>[3x]GSPSSQGQHKHKYHFQKTFTVSQAGNCRIMAYCDALSCLVISQPSPQASFLPGFGVKMLSTANMKSSQYIPMHGKQIRGLAFSSYLRGLLLSASLDNTIKLTSLETNTVVQTYNAGRPVWSCCWCLDEANYIYAGLANGSILVYDV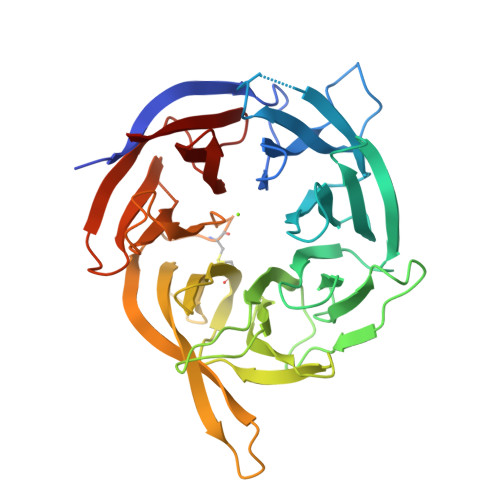RNTSSHVQELVAQKARCPLVSLSYMPRAASAAFPYGGVLAGTLEDASFWEQKMDFSHWPHVLPLEPGGCIDFQTENSSRHCLVTYRPDKNHTTIRSVLMEMSYRLDDTGNPICSCQPVHTFFGGPTCKLLTKNAIFQSPENDGNILVCTGDEAANSALLWDAASGSLLQDLQTDQPVLDICPFEVNRNSYLATLTEKMVHIYKWE> MASATTSSKNGKPLVVVYGDYKCPYCKELDEKVMPKLRKNY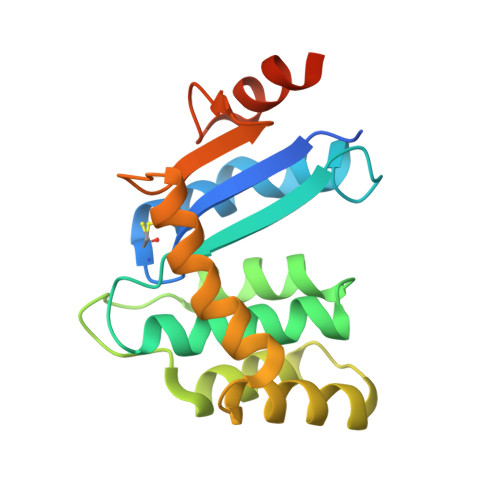IDNHKVEYQFVNLAFLGKDSIVGSRASHAVLMYAPKSFLDFQKQLFAAQQDQNKEWLTKELLDKHIKQLHLDKETENKIIKDYKTKDSKSWKAAEKDKKIAKDNHIKTTPTAFINGEKVEDPYDYESYEKLLKDKIKLEHHHHHH N-benzyl-2-({N-[2-(1H-indol-3-yl)ethyl]glycyl}amino)-4-phenylthiophene-3-carboxamide 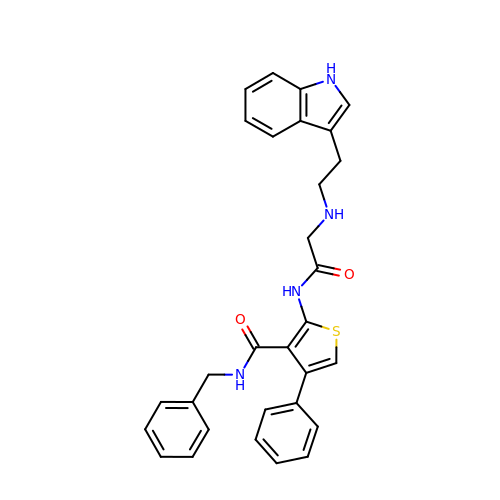| C30 H28 N4 O2 S | NZMGUKNNKODUOD-UHFFFAOYSA-N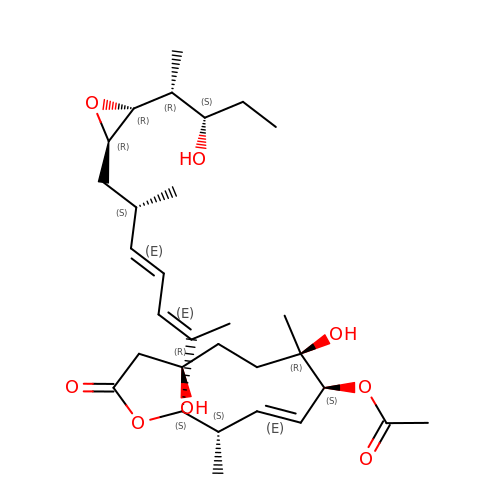[(2~{S},3~{S},4~{E},6~{S},7~{R},10~{R})-3,7-dimethyl-2-[(2~{E},4~{E},6~{S})-6-methyl-7-[(2~{R},3~{R})-3-[(2~{R},3~{S})-3-oxidanylpentan-2-yl]oxiran-2-yl]hepta-2,4-dien-2-yl]-7,10-bis(oxidanyl)-12-oxidanylidene-1-oxacyclododec-4-en-6-yl] ethanoate | C30 H48 O8 | SDOUORKJIJYJNW-QHOUZYGJSA-N>[2x]MCELYSKRDTLGLRKKHIGPSCKVFFASDPIKIVRAQRQYMFDENGEQYLDCINNVAHVGHCHPGVVKAALKQMELLNTNSRFLHDNIVEYAKRLSATLPEKLSVCYFTNSGSEANDLALRLARQFRGHQDVITLDHAYHGHLSSLIEISPYKFQKGKDVKKEFVHVAPTPDT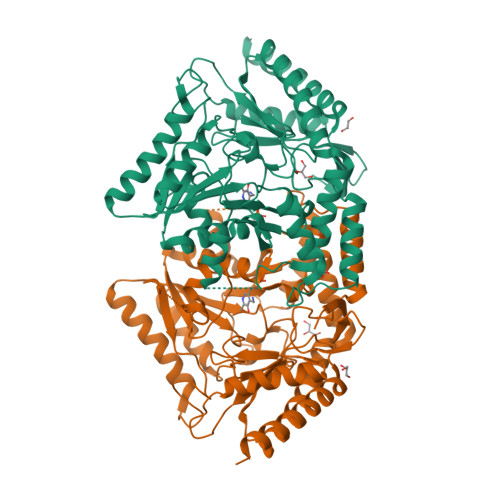YRGKYREDHADSASAYADEVKKIIEDAHNSGRKIAAFIAESMQSCGGQIIPPAGYFQKVAEYVHGAGGVFIADEVQVGFGRVGKHFWSFQMYGEDFVPDIVTMGKPMGNGHPVACVVTTKEIAEAFSSSGMEYFNTYGGNPVSCAVGLAVLDIIENEDLQGNAKRVGNYLTELLKKQKAKHTLIGDIRGIGLFIGIDLVKDHLKRTPATAEAQHIIYKMKEKRVLLSADGPHRNVLKIKPPMCFTEEDAKFMVDQLDRILTVLEEAMGTKTESVTSENTPCKTKMLKEAHIELLRDSTTDSKENPSRKRNGMCTDTHSLLSKRLKT L-deoxythymidine | C10 H14 N2 O5 | 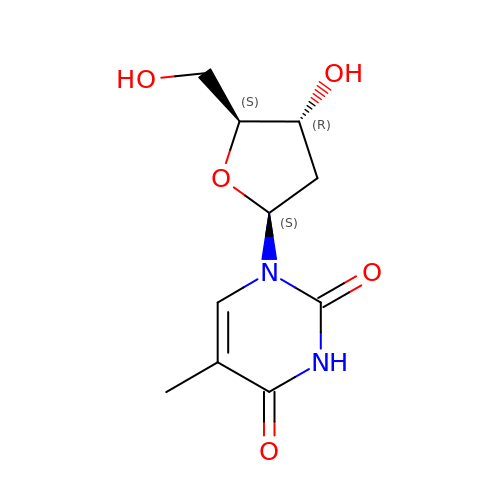IQFYYKKMVGJFEH-CSMHCCOUSA-N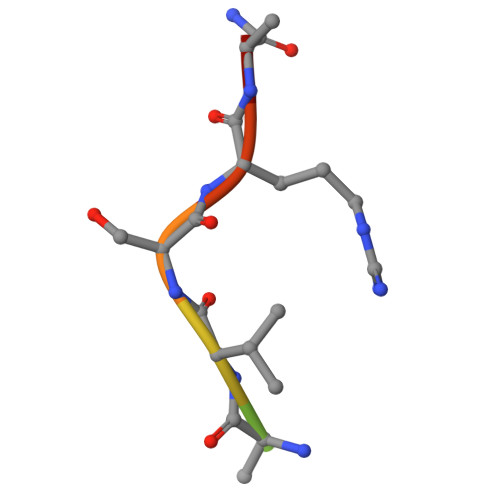> KKVAVSRAA>MKHQHQHQHQHQHQQPLQPLNEEFRPEMLQGKKVIVTGASKGIGREMAYHLAKMGAHVVVTARSKE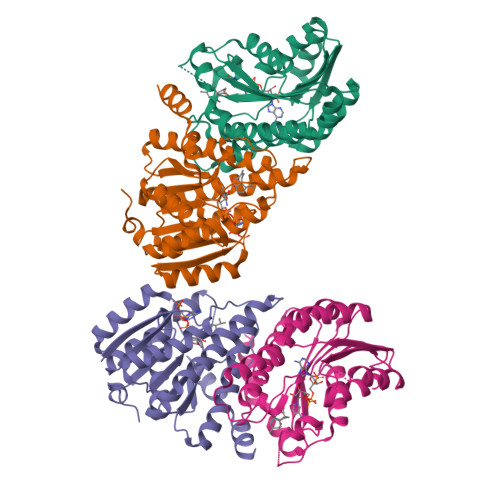TLQKVVSHCLELGAASAHYIAGTMEDMTFAEQFVAQAGKLMGGLDMLILNHITNTSLNLFHDDIHHVRKSMEVNFLSYVVLTVAALPMLKQSNGSIVVVSSLAGKVAYPMVAAYSASKFALDGFFSSIRKEYSVSRVNVSITLCVLGLIDTETAMKAVSGIVHMQAAPKEECALEIIKGGALRQEEVYYDSSLWTTLLIRNPSRKILEFLYSTSYNMDRFINK[4x]> MIWTGLLVGFLFGIVLQRGRICFNSAFRDVLLFKDNYLFKLAVFTLALEMILFVLLSQVGLMQMNPKPLNLVGNIIGGFVFGLGMVLAGGCASGVTYRVGEGLTTAWFAALFYGLGAYATKSGAFSWWLSWVGQFKSPLSVEESAYYVKGAGPTISSVLGLNPWIPALVIAALFILWAFGTKTTSR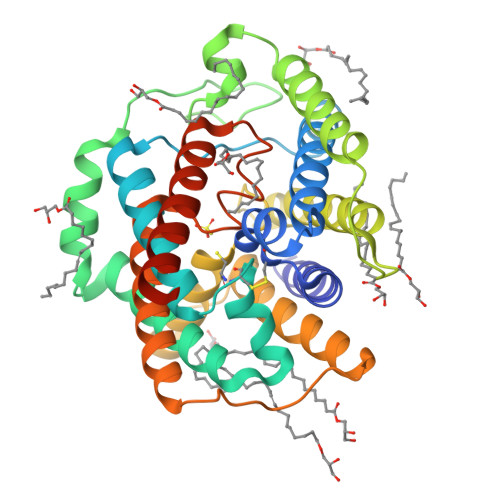ETKFNWKIASVCLALVAGLGFITSTLSGRKYGLGITGGWINLFQGFLTNSPLNWEGLEIVGIILGAGVAAAVAGEFKLRMPKNPVTYLQVGIGGLLMGIGAVTAGGCNIGHFLTGVPQLALSSWLASIFFILGNWTMAWILFLESSGENLYFQ> SNAGPFIRPSYAQAGALKVGLLLPYSGTYAPLGEAITRGLELYVQSQGGKLGGRSISFVKVD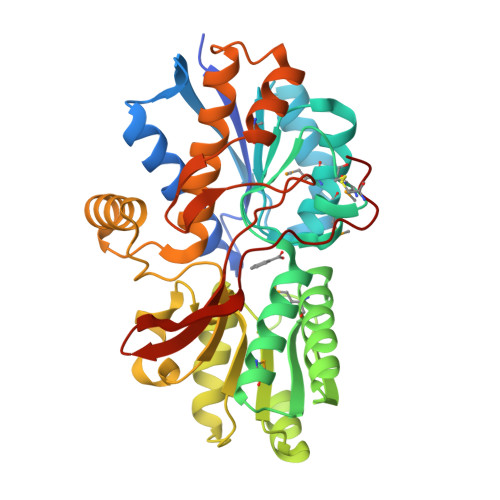DESAPPKATELTTKLIQSEKADVLIGTVHSGVAMAMVKIAREDGIPTIVPNAGADIITRAMCAPNVFRTSFANGQIGRATGDAMIKAGLKKAVTVTWKYAAGEEMVSGFKKSFTAGKGEVVKDITIAFPDVEFQSALAEIASLKPDCVYAFFSGGGALKFIKDYAAANLGIPLWGPGFLTDGVEAAAGPAGDGIKTVLHYVSDLDNAENQAFVKSFEAAYKIPPDVFAVQGWDAGQLLDAGVKAVGGDVAKRKELNAAMAAASFASPRGPFKLSAAHNPVQNFYLRELKGGKSVNLGLAAPAVADEAIGCKLS>[2x]MATQMRLTDTNLLEVLNSEEYSGVLKEFREQRYSKKAILYTPNTERNLVFLVKSGRVRVYLAYEDK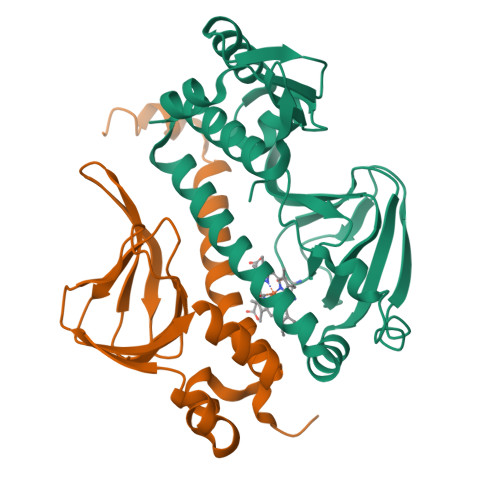EFTLAILEAGDIFCTHTRAFIQAMEDTTILYTDIRNFQNIVVEFPAFSLNMVKVLGDLLKLLLTIINGLVFKDARLRLAEFLVQAAMDTGLKVPQGIKLELGLNTEEIALMLGTTRQTVSVLLNDFKKMGILERVNQRTLLLKDLQKLKEFSSGV Central to these functions, RAD52 promotes the annealing of complementary single-stranded DNA (ssDNA)8,9 and provides an alternative to BRCA2/RAD51-dependent homologous recombination repair. Instead, cryo-electron microscopy and biochemical analyses revealed that ssDNA annealing is driven by RAD52 open rings in association with replication protein-A (RPA). RPA associates with RAD52 at the site of ring opening with critical interactions occurring between the RPA-interacting domain of RAD52 and the winged helix domain of RPA2. Our studies provide structural snapshots throughout the annealing process and define the molecular mechanism of ssDNA annealing by the RAD52–RPA complex.

One possibility is that this domain is flexible before interaction with ssDNA, enabling rapid and tight association with ssDNA. To determine the validity of this hypothesis, the structure of the RAD52-OR bound to ssDNA (2.3 Å) was solved. An analysis of the RAD52–ssDNA complex revealed that the DBD was stabilized as ssDNA bound into the positively charged groove on the outside of the RAD52 ring. Atomic models of the RAD52–ssDNA complex show that ssDNA sits in a positively charged channel around the ring. In the RAD52-OR–ssDNA complex, the ssDNA could be visualized from the second to the seventh RAD52 subunit. There were four ssDNA nucleotides per RAD52 subunit, consistent with the observed four-nucleotide pattern of hypersensitivity to hydroxyl radicals. Topological analysis of the structure revealed that the bound ssDNA was stretched non-uniformly, such that each quartet stack adopted the length of B-form duplex DNA. Arg153 coordinated the phosphate backbone of the two central nucleotides, whereas Arg55 and Lys152 coordinated the phosphate backbone between two quartet stacks. The Mg2+, which is required for RAD52–ssDNA interactions, and the surrounding water molecules were coordinated by Glu145, Asp149 and Glu140 residues from the neighbouring subunit. In agreement, using focused 3D classification analysis, we found a subclass of RAD52–ssDNA particles that exhibited a low-resolution density across the site of ring opening corresponding to the C-terminal domain of RAD52.

>[9x]MSGTEEAILGGRDSHPAAGGGSVLCFGQCQYTAEEYQAIQKALRQRLGPEYISSRMAGGGQKVCYIEGHRVINLANEMFGYNGWAHSITQQNVDFVDLNNGKFYVGVCAFVRVQLKDGSYHEDVGYGVSEGLKSKALSLEKARKEAVTDGLKRALRSFGNALGNCILDKDYLRSLNKLPRQLPLEVDLTKAKRQDLEPSVEEARYNSCRPNMALGHPQLQQVTSPSRPSHAVIPADQDCSSRSLSSSAVESEATHQRKLRQKQLQQQFRERMEKQQVRVSTPSAEKSEAAPPAPPVTHSTPVTVSEPLLEKDFLAGVTQELIKTLEDNSEKWAVTPDAGDGVVKPSSRADPAQTSDTLALNNQMVTQNRTPHSVCHQKPQAKSGSWDLQTYSADQRTTGNWESHRKSQDMKKRKYDPS> MKFILAEKFTFDPLSNTLIDKEDSEEIIRLGSNESRILWLLAQRPNEVISRNDLHDFVWREQGFEVDDS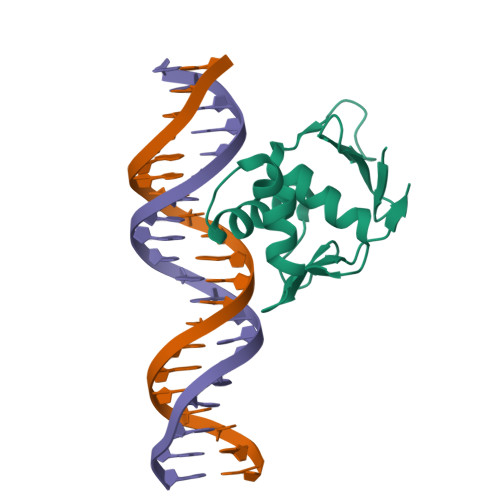SLTQAISTLRKMLKDSTKSPQYVKTVPKRGYQLIARVETV>[8x]MAVELGVLLVRPRPGTGLGRVMRTLLLVLWLATRGSALYFHIGETEKKCFIEEIPDETMVIGNYRTQLYDKQREEYQPATPGLGMFVEVKDPEDKVILA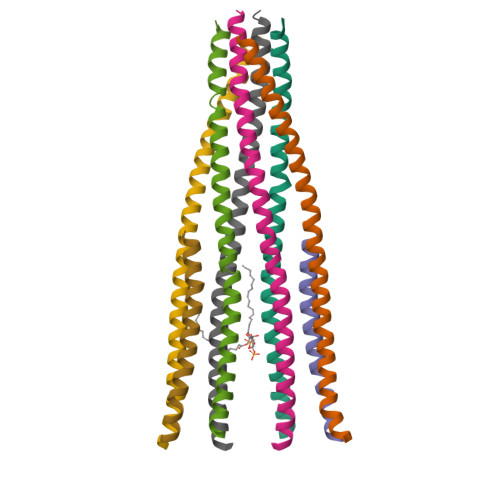RQYGSEGRFTFTSHTPGEHQICLHSNSTKFSLFAGGMLRVHLDIQVGEHANDYAEIAAKDKLSELQLRVRQLVEQVEQIQKEQNYQRWREERFRQTSESTNQRVLWWSILQTLILVAIGVWQMRHLKSFFEAKKLV> MDGLELRKLGEVSWEEEAEISGSSARYDVTLSEQGEFKLLSEEKVPWD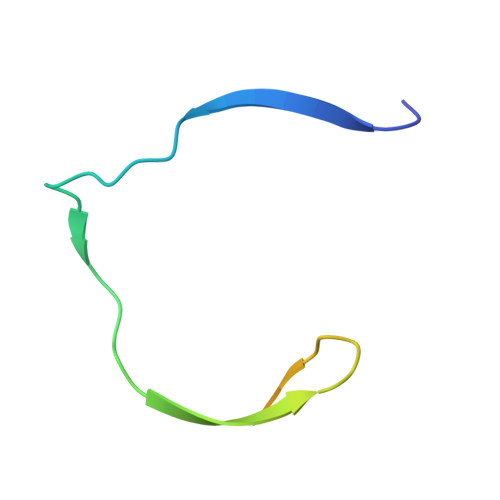GGGGSGGGG> MYNTISITVVDADDVG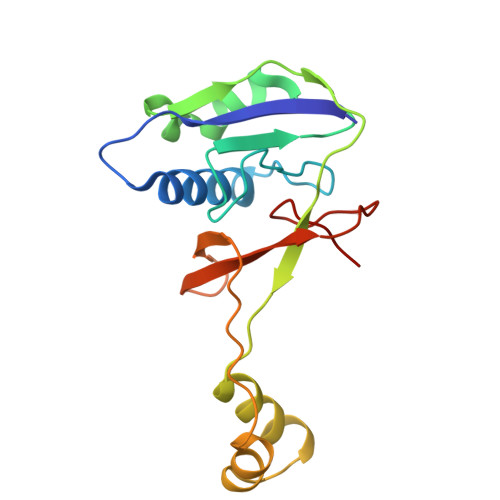VNFVVSKVLSTLHNKGIFNGEVGVTFPRMDKNVGDIITLFSKTGVDRKVLTSTLNTLTDFIHIGKPKEADKVKTYRKVDTKSKGKLIRRCIKRKGVSAETAESLYGNYKGEKCKLPYIVVNSKSTGQRFSMFLEECENSEKFNSYGLCIVSC> PPTKKVLDENGQSINGKSVLPNATLDYVAKQNFSQYKGIKASAEAIAKGFAFVDQPNEALAELTVKSIKASNGDDVSSLLEMRHVLSKDTLDQKLQSLIKEAGISPVGEFYMWTAKDPQAFYKAYVQKGLDITYNLSFKVKKEFTKGQIKNGVAQIDFGNGYTGNIVVNDLTTPEVHKD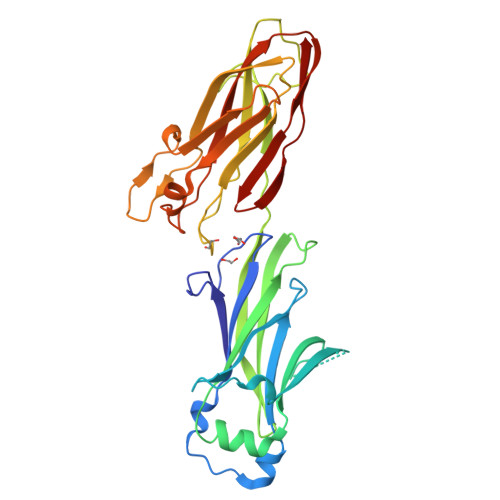VLDKEDGKSINNGTVKLGDEVTYKLEGWVVPANRGYDLFEYKFVDHLQHTHDLYLKDKVVAKVAITLKDGTVIPKGTNLVQYTETVYNKETGRYELAFKADFLAQVSRSSAFGADDFIVVKRIKAGDVYNTADFFVNGNKVKTETVVTHT3-[2-methyl-6-(pyrazin-2-ylamino)pyrimidin-4-yl]-N-(1H-pyrazol-3-yl)imidazo[1,2-b]pyridazin-2-amine 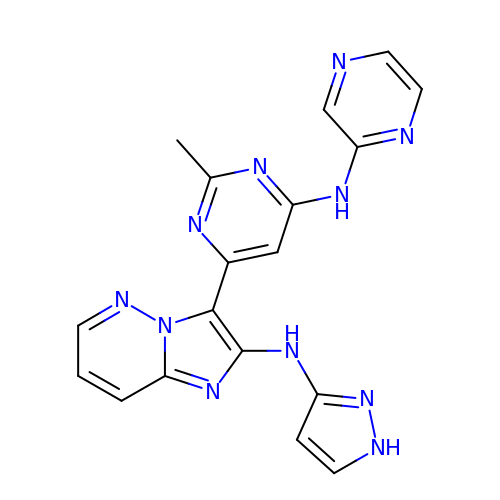| C18 H15 N11 | ABQRVDGZZXHLLT-UHFFFAOYSA-N> QFAKPEDA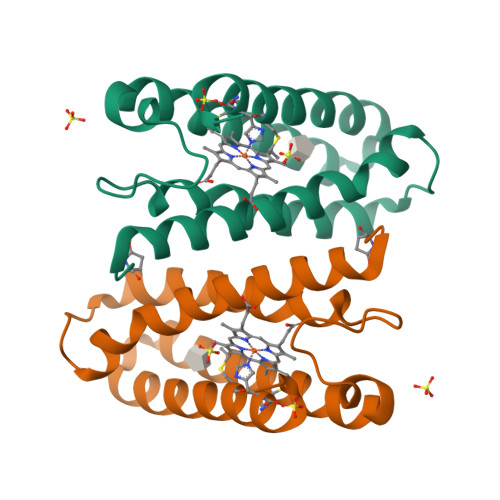VKYRQSAFTLMASHFGRMTPVVKGQAPYDAAQIKANVEVLKTLSALPWAAFGPGTEGGDARPEIWSDAASFKQKQQAFQDNIVKLSAAADAGDLDKLRAAFGDVGASCKACHDAYRKK[(7~{S})-1-bromanyl-6,6-bis(oxidanyl)-4-phenyl-5,7,8,9-tetrahydrobenzo[7]annulen-7-yl]azanium | C17 H19 Br N O2 | 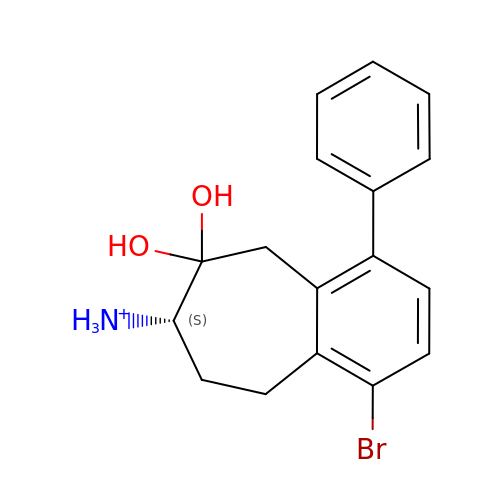YMWOHZAVFJCVSC-INIZCTEOSA-O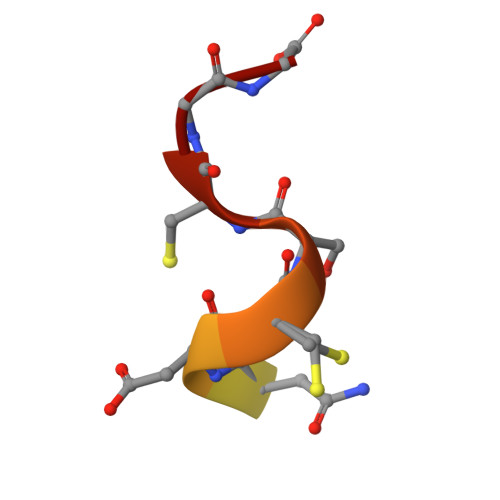> EDSHKESNDCSCGG>[4x]MGHHHHHHHHHHSSGHIEGRHMMATNLRGVMAALLTPFDQQQALDKASLRRLVQFNIQQGIDGLYVGG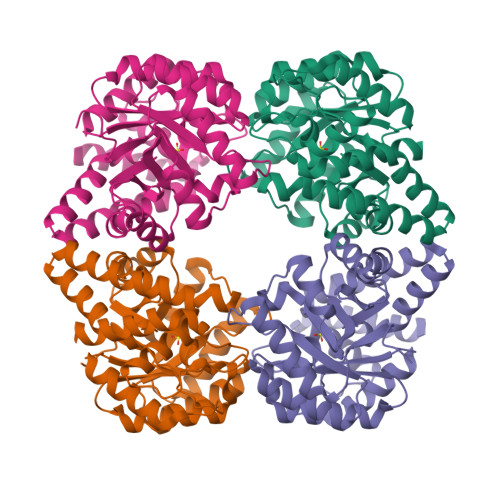STGEAFVQSLSEREQVLEIVAEEAKGKIKLIAHVGCVSTAESQQLAASAKRYGFDAVSAVTPFYYPFSFEEHCDHYRAIIDSADGLPMVVYNIPALSGVKLTLDQINTLVTLPGVGALKQTSGDLYQMEQIRREHPDLVLYNGYDEIFASGLLAGADGGIGSTYNIMGWRYQGIVKALKEGDIQTAQKLQTECNKVIDLLIKTGWFRGLKTVLHYMDVVSVPLCRKPFGPVDEKYLPELKALAQQLMQERG>[2x]MA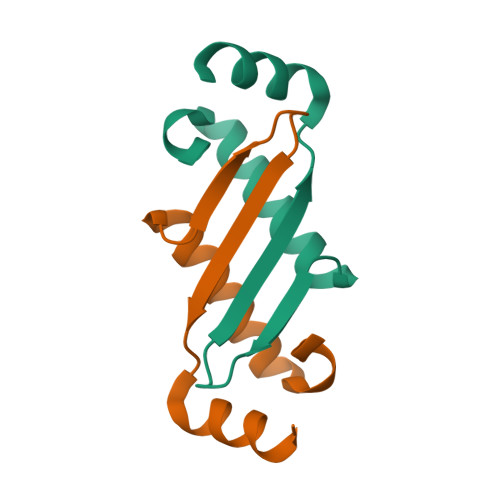HHHHHHTEDDVRHHFTPSERQLCLSSIQTAFNQGAGTCTLSDSGRISYTVEFSLPTHHTVRLIRVTASPSA> MTKALFFD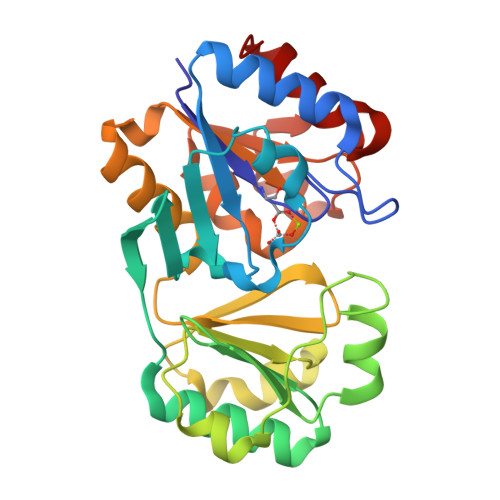IAGTLVSFETHRIPSSTIEALEAAHAKGLKIFIATGRPKAIINNLSELQDRNLIDGYITMNGAYCFVGEEVIYKSAIPQEEVKAMAAFCEKKGVPCIFVEEHNISVCQPNEMVKKIFYDFLHVNVIPTVSFEEASNKEVIQMTPFITEEEEKEVLPSIPTCEIGRWYPAFADVTAKGDTKQKGIDEIIRHFGIKLEETMSFGDGGNDISMLRHAAIGVAMGQAKEDVKAAADYVTAPIDEDGISKAMKHFGII> MHHHHHHHHAAAGLVPRGSMSQTSTLKGQCIAEFLGTGLLIFFGVGCVAALKVAGASFGQWEI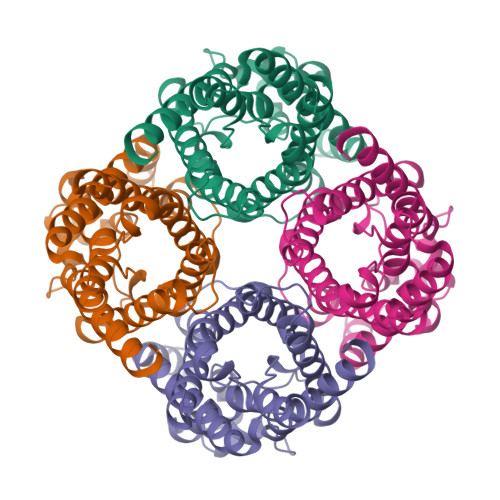SVIWGLGVAMAIYLTAGVSGAHLNPAVTIALWLFACFDKRKVIPFIVSQVAGAFCAAALVYGLYYNLFFDFEQTHHIVRGSVESVDLAGTFSTYPNPHINFVQAFAVEMVITAILMGLILALTDDGNGVPRGLAPLLIGLLIAVIGASMGPLTGFAMNPARDFGPKVFAWLAGWGNVAFTGGRDIPYFLVPLFGPIVGAIVGAFAYRKLIGRHLPCDICVVEEKETTTPSEQKASL CARBOXYMETHYL COENZYME *A | C23 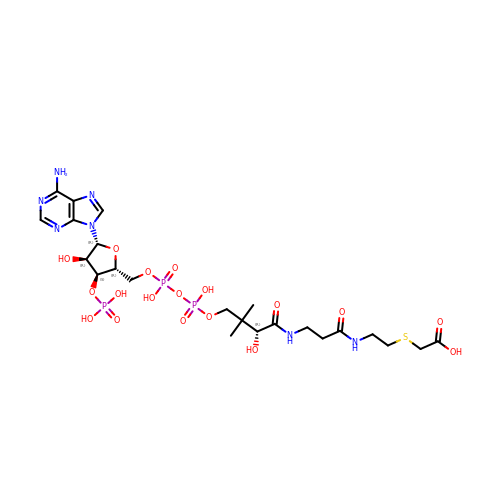H38 N7 O18 P3 S | OBUOSIHPWVNVJN-GRFIIANRSA-N Channelrhodopsins (ChRs) are light-gated cation channels first identified as sensory photoreceptors in green algae. ChRs consist of seven transmembrane helices and a retinal chromophore covalently attached to a conserved lysine residue via a Schiff base linkage. As in the well-studied bacterial proton pump bacteriorhodopsin (BR), light absorption triggers all-trans to 13-cis isomerization of the retinal, and induces the transitions of optically distinguishable intermediates that lead to channel opening and closing (photocycle process) (Kuhne et al., 2019; Bamann et al., 2010; Bamann et al., 2008). We used a chimeric construct between Chlamydomonas reinhardtii ChR1 (CrChR1) and ChR2 (CrChR2) for the TR-SFX experiments (hereafter referred to as C1C2) (Kato et al., 2012), which has normal ChR1 photocycle properties (Hontani et al., 2017; Inaguma et al., 2015).

C1C2 yielded high-density microcrystals that diffracted XFEL to about 2.3 Å at SACLA. The dark state structure of C1C2 determined at SACLA is almost the same as the previous structure solved by the synchrotron analysis, including the chromophore retinal, the interhelical interactions of the inner and central gates, and the extracellular water access channel in the dark state (Hontani et al., 2017). (c) The structure of dark state C1C2 determined by serial femtosecond crystallography. A water accessible cavity is illustrated, with the putative ion pathway indicated by an arrow. The five glutamic acid residues lining the ion pore (E1–5) and the two counterion residues (Ci1 and Ci2) are indicated by sticks, and the three constriction sites, the inner, central, and outer gates, are enclosed in boxes. TM7 contributes essentially to the ‘central gate’, in which Asn297 forms hydrogen bond interactions with Ser102 (TM1) and Glu129 (TM2). The intracellular end of TM3 shapes the ‘inner-gate’, in which His173 forms ionic interactions with Arg307 in TM7 and Glu121 and Glu122 in TM2. The inner gate formed by Glu121, Glu122, His173, and Arg307 prevents water influx in the initial dark-adapted state. The crystal packing of C1C2 shows minimal packing interactions, as compared to the CrChR2 crystal packing.

> MSRRPWLLALALAVALAAGSAGASTGSDATVPVATQDGPDYVFHRAHERMLFQTSYTLENNGSVICIPNNGQCFCLAWLKSNGTNAEKLAANILQWITFALSALCLMFYGYQTWKSTCGWEEIYVATIEMIKFIIEYFHEFDEPAVIYSSNGNKTVWLRYAEWLLTCPVILIHLSNLTGLANDYNKRTMGLLVSDIGTIVWGTTAALSKGYVRVIFFLMGLCYGIYTFFNAAKVYIEAYHTVPKGRCRQVVTGMAWLFFVSWGMFPILFILGPEGFGVLSVYGSTVGHTIIDLMSKNCWGLLGHYLRVLIHEHILIHGDIRKTTKLNIGGTEIEVETLVEDEAEAGAVSSEDLYFQ> GPEFLSNKQTHWY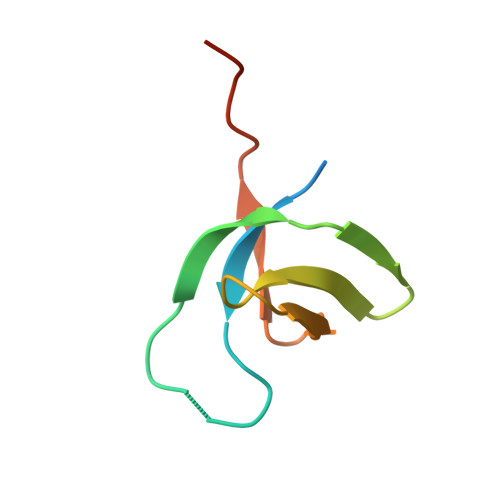YFKLPGLNSRQWKGPQEALQEAAGAALIPVSASSAQWIPWRLLKRAACPRPVGGPA> LKESPSGYLRSGEGDTGCGELVWVGEPLTLRTAETITGKYGVWMRDPKPTYPYTQETTWRIDTVGTDVRQVFEYDLISQFMQGYPSKVHILPRPLESTGAVVYSGSLYFQGAESRTVIRYELNTKTVKAEKEIPGAGYHGQFPYSWGGYTDIDLAVDEAGLWVIYSTDEAKGAIVLSKLNPENLELEQTWETNIRKQSVANAFIICGTLYTVSSYTSADATVNFAYDTGTGISKTLTIPFKNRYKYSSMIDYNPLEKKLFAWDNLNMVTYDIKLSKM

Inherited missense mutations in the myocilin (MYOC) gene, within its olfactomedin (OLF) domain, constitute the strongest genetic link to primary open-angle glaucoma via a toxic gain of function, and thus MYOC is an attractive precision-medicine target. Myocilin has no known function, and there is no glaucoma phenotype in Myoc knockout mice or in individuals with a homozygous N-terminal truncation mutation or hemizygous deletion of MYOC, but rare non-synonymous coding mutations lead to toxic intracellular sequestration of misfolded myocilin. However, not all mutations in MYOC cause glaucoma, and common variants are expected to be neutral polymorphisms. Among the common features associated with pathogenic myocilin misfolding, we demonstrate that a single metric, OLF thermal stability, can robustly segregate benign from early-onset disease variants.

Illustrative of this latter group is E352K, a variant documented in gnomAD as appearing predominantly in the African or African American population. E352K has been computationally predicted to be pathogenic and has been documented both in primary open-angle glaucoma (POAG) patients and in control groups, yet exhibits WT-like secretion. Modestly lower levels than WT were detected for T293K, E352K, K398R, N420Y and A427T. Structural integrity was further confirmed by high-resolution crystal structures, which were solved for 11 OLF variants. No gross changes from WT OLF were detected for the structures of T293K, R296H, L303I, V329M, S331L, E352K, T353I, K398R, A445V, V449I or K500R, indicating that these mutations are accommodated within the native five-bladed β-propeller fold and do not perturb the dinuclear calcium-containing site. Similarly, the finding that E352K does not exhibit characteristics of misfolding is consistent with the later age of diagnosis of glaucoma for patients with the E352K variant and a lack of clear Mendelian inheritance pattern. Most of the patients with E352K are of African or African American ancestry, a group more prone to developing POAG. Our findings rule out misfolding of E352K as causal for this higher glaucoma risk and suggest that other mechanisms are likely at play.> GHMDTPVLTPTEAAVLRELRLHRPQLPLDTLLFTDPNKDPDDVVTYTIAKQLQADGFLRLTDVVVTLGDADMRSQRAQLAKGVFDRLALPDVRVARGQDYPMTSTQAREHSKFLAEGAALRAAPDAVHTDGVRAMCERLATSPHKLGMVVIAGMTDASALLAEAGDLVREKVASITIMGGIDPARDADGLVQPDTRAYNNATDIHAARALYRRAQQLGIPLRILTKEAAYKAAVPPAFYEGIARNGHPVGEYLRDVQKNALKGLWEGIQANLIPGLDTAWFFRTFVAAQPQDPVAADQQGALSFDAIWPQVTKLNLYDPLTLL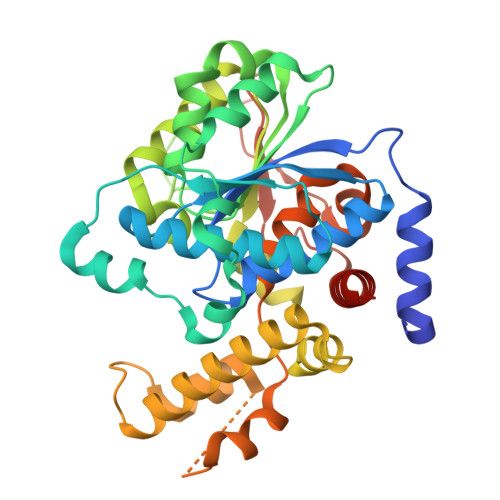AALPGTARLLFQPTPMHREGASPVEHVGHAEVVRPEKARLLLSALAKAALVQQDEG>[7x]GSP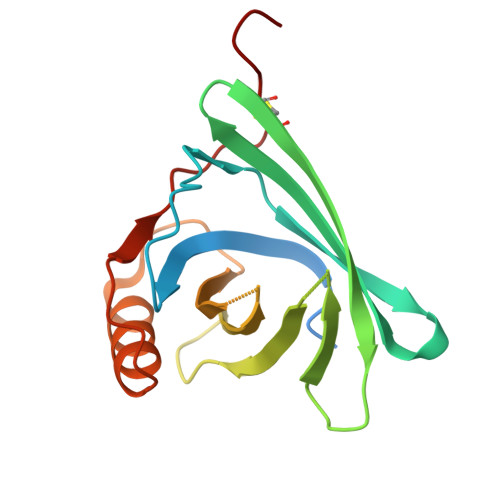GIPGQDTPALGKDTVAVSGKWYLKAMTADQEVPEKPDSVTPMILKAQKGGNLEAKITMLTNGQCQNITVVLHKTSEPGKYTAYEGQRVVFIQPSPVRDHYILYAEGELHGRQIRMAKLLGRDPEQSQEALEDFREFSRAKGLNQEILELAQSETCSPGGQ>MKTLTAILISSVFASAAASAQTANTPTPTAGVQAFLNVLNSGKGKPMEQMTPQEARQVLIGAQQGAKLPPAQVSEKTIQVNGQAIKLKIVKPENASGTLPAFMFFHGGGWVLGDFPTHERLIRDLVRASGAAAVYVDYTPSPEAHFPVAINQAYEATKWVAEHGQEIGVDGSRLGLVGNSVGGNMVASVALQAKQFNGPKIRYNVMLWPVTDANFDTASYNQFENGYFLSKNMMKWFWDNYTTSAADRNNILASPLRASTAQLKGFPETLIQTAELDVLRDEGEAFGRKLDAAGVPVTVTRYNGMIHDYGLLNPLSQEPTV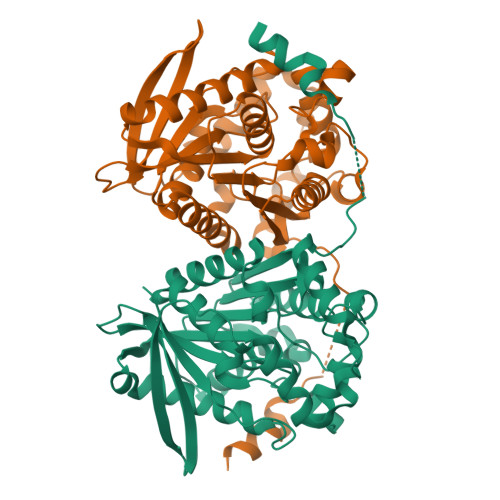KVALEQAGAALHEHLK[2x]> MDFETGEHQYQYKDILSVFEDAFVDNFDCKDVQDMPKSILSKEEIDHIIM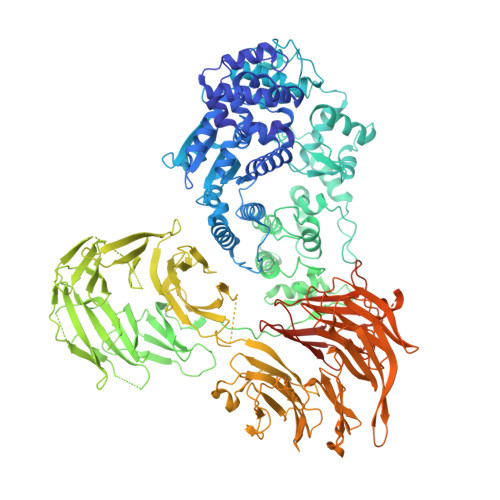SKDAVSGTLRLFWTLLSKQEEMVQKFVEEVLRINYKFLMSPIKTEQRQPSMMTRMYIEQRDRLYNDNQVFAKYNVSRLQPYLKLRQALLELRPAKNVLIDGVLGSGKTWVALDVCLSYKVQCKMDFKIFWLNLKNCNSPETVLEMLQKLLYQIDPNWTSRSDHSSNIKLRIHSIQAELRRLLKSKPYENCLLVLLNVQNAKAWNAFNLSCKILLTTRFKQVTDFLSAATTTHISLDHHSMTLTPDEVKSLLLKYLDCRPQDLPREVLTTNPRRLSIIAESIRAGLATWDNWKHVNCDKLTTIIESSLNVLEPAEYRKMFDRLSVFPPSAHIPTILLSLIWFDVIKSDVMVVVNKLHKYSLVEKQPKESTISIPSIYLELKVKLENEYALHRSIVDHYNIPKTFDSDDLIPPYLDQYFYSHIGHHLKNIEHPERMTLFRMVFLDFRFLEQKIRHDSTAWNASGSILNTLQQLKFYKPYICDNDPKYERLVNAILDFLPKIEENLICSKYTDLLRIALMAEDEAIFEEAHKQVQRFDDRVWFTNHGRFHQHRQIINLGDNEGRHAVYLHNDFCLIALASGQILLTDVSLEGEDTYLLRDESDSSDILRMAVFNQQKHLITLHCNGSVKLWSLWPDCPGRRHSGGSKQQLVNSVVKRFIGSYANLKIVAFYLNEDAGLPEANIQLHVAFINGDVSILNWDEQDQEFKLSHVPVLKTMQSGIRCFVQVLKRYYVVCTSNCTLTVWDLTNGSSNTLELHVFNVENDTPLALDVFDERSKTATVLLIFKYSVWRLNFLPGLSVSLQSEAVQLPEGSFITCGKRSTDGRYLLLGTSEGLIVYDLKISDPVLRSNVSEHIECVDIYELFDPVYKYIVLCGAKGKQVVHVHTLRSVSGSNSHQNREIAWVHSADEISVMTKACLEPNVYLRSLMDMTRERTQLLAVDSKERIHLIKPAISRISEWSTITPTHAASNCKINAISAFNDEQIFVGYVDGVIIDVIHDTALPQQFIEEPIDYLKQVSPNILVASAHSAQKTVIFQLEKIDPLQPNDQWPLMMDVSTKYASLQEGQYIILFSDHGVCHLDIANPSAFVKPKDSEEYIVGFDLKNSLLFLAYENNIIDVFRLIFSCNQLRYEQICEEEIAQKAKISYLVATDDGTMLAMGFENGTLELFAVENRKVQLIYSIEEVHEHCIRQLLFSPCKLLLISCAEQLCFWNVTHMRNNQLEREQKRRRSRRHKQHSVTQEDAVDAAPIAADIDVDVTFVADEFHPVNRGTAELWRNKRGNAIRPELLACVKFVGNEARQFFTDAHFSHFYAIDDEGVYYHLQLLELSRLQPPPDPVTLDIANQYEDLKNLRILDSPLMQDSDSEGADVVGNLVLEKNGGVARATPILEEASSHHHHHH> GSHMSGRAPAPVAATTQPKLVTGDITSTDQSGTNLFFGKKIVRNARGAIMKVDRTWPAAVPAPLPDVRADSSTRMLLGPVVDLAVNEHPEGVFYRIPALATASNGDLLASYDLRPGSAGDAPNPNSIVQRRSRDNGRTWGPQTVIHAGTPGRRKVGYSDPSYLVDPATGRILNFHVKSYDRGFATSEVGTDPDDRHVLHAEVSTSTDNGHTWTHRDITREITSDPTTRTRFVASGQGIALLHGPHAGRLIAQMTVRNSVGQQAQSIYSDDHGITWHAGNPVGRMMDENKVVELSDGTLMLNSRDAARSGRRKVAYSQDGGLTWGPVK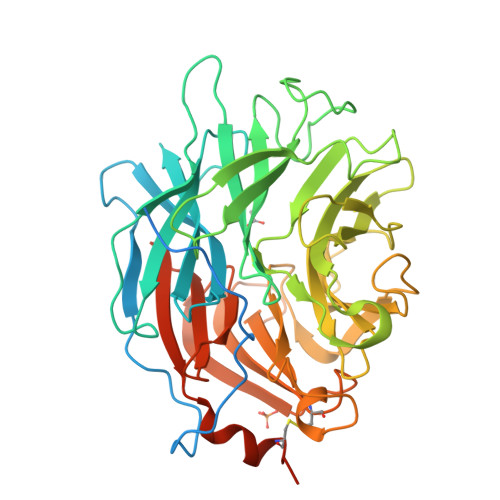LVDDLIDPTNNAQIIRAYPNARAGSAKARILLFTNARNATERVNGTLSVSCDDGRTWVSHQTYMPGEVGYTTAAVQSDGALGVLWERDGIRYSTIPMGWLNSVCPLAPSGRPTSGKPTSGTSLPPTAT> MTFTKACSVDEVPPGEALQVSHDAQKVAIFNVDGEFFATQDQCTHGEWSLSEGGYLDGDVVECSLHMGKFCVRTGKVKSPPPCEPLKVYPIRIEGRDVLV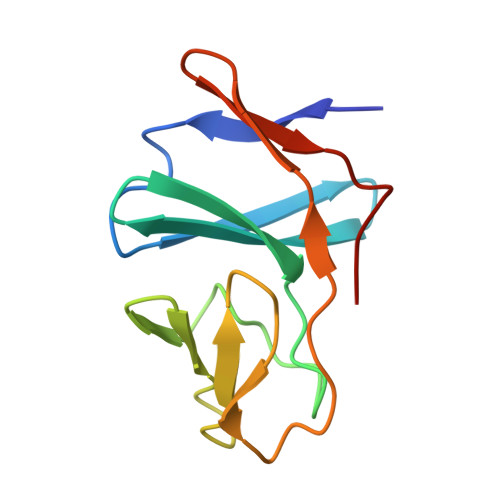DFSRAALHA>MGSDKIHHHHHHENLYFQGMTEKSQEPTAALDAEQVAAYLSQHPEFFVEHDELIPELRIPHQPGDAVSLVERQVRLLRERNIEMRHRLSQLMDVARENDRLFDKTRRLVLDLLDATSLEDVVSTVEDSLRHEFQVPYVSLILFSDSSVSVGRSVSSAEAHQAIGGLLSGGKTVCGVLRPHELAFLFGESDRDEIGSAAVVSLSFQGLH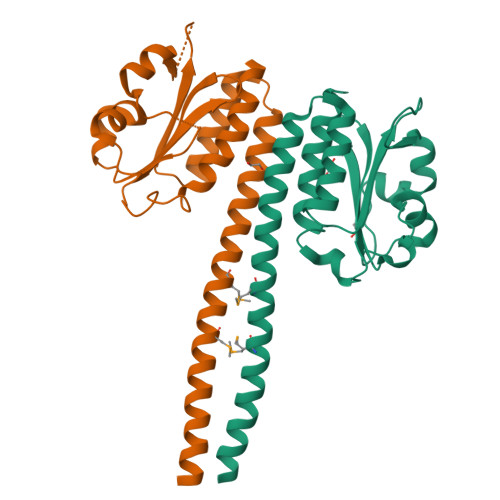GVLAIGSPDPQHYKSSLGTLFLGYVAEVLARVLPRFSSPLRSVR[2x]> MYSKIKISGTIEVVTGLHIGGGGESSMIGAIDSPVVRDLQTKLPIIPGSSIKGKMRNLLAKHFGLKMKQESHNQDDERVLRLFGSSEKGNIQRARLQISDAFFSEKTKEHFAQNDIAYTETKFENTINRLTAVANPRQIERVTRGSEFDFVFIYNVDEESQVED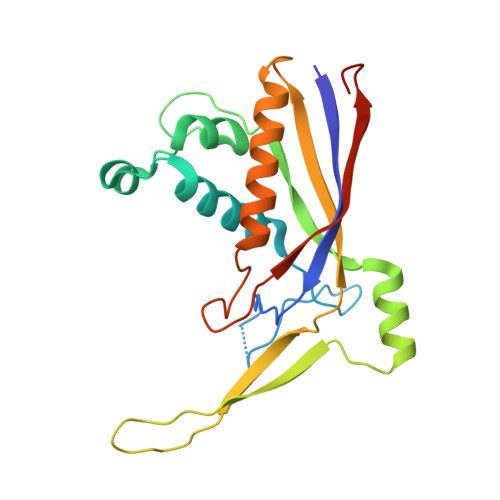DFENIEKAIHLLENDYLGGGGTRGNGRIQFKDTNIETVVGEYDSTNLKIK> SGISLDNSYKMDYPEMGLCIIINNKNFHKSTGMTSRSGTDVDAANLRETFRNLKYEVRNKNDLTREEIVELMRDVSKEDHSKRSSFVCVLLSHGEEGIIFGTNGPVDLKKITNFFRGDRCRSLTGKPKLFIIQACRGTELDSGIETDSGVDDDMACHKIPVEADFLYAYSTAPGYYSWRNSKDGSWFIQSLCAMLKQ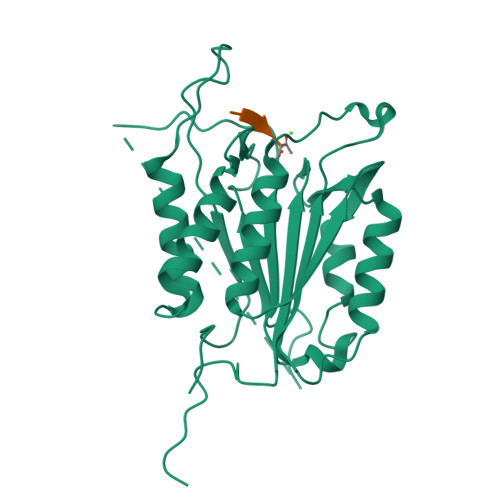YADKLEFMHILTRVNRKVATAFESFSFDATFHAKKQIPCIVSMLTKELYFYHH(2S)-2-{[(R)-{[(2R,3S,4R,5R)-5-(6-amino-9H-purin-9-yl)-3,4-dihydroxyoxolan-2-yl]methoxy}(hydroxy)phosphoryl]amino}propanoic 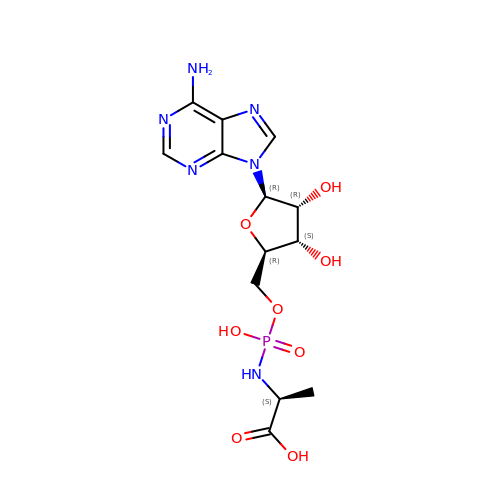acid (non-preferred name) | C13 H19 N6 O8 P | FRQHIZTYMNUOJX-MACXSXHHSA-N>[10x]MAHHHHHHMARNYAY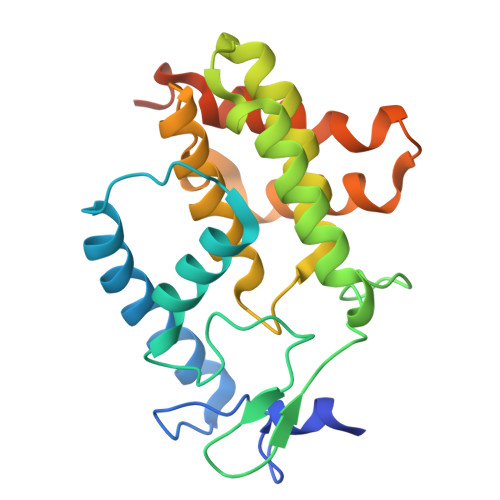PHMNTLKNKHNIMSTKKLAHVCEHYAKKAIINLNKEPLPQKFDSSYLKYIHQRLFESTFEWAGYTRDFSFTFDDGTVAEMPMMKVPNLDIFYVQGNDIQENLKKFDQLLASKNNLQGLSREEFVDEAAKLFVFLNSIAPFRAGNEPTQRVFFEKLAEAAGHQLDFSVATEKRIMRACIDGMTLKDNMAYKEMKSLFEDISDPKKIAALKNFLRRIPRLERERLNDE> MLVLVAPGQGAQTPGFLTDWLALPGAADRVAAWSDAIGLDLAHFGTKADADEIRDTSVAQPLLVAAGILSAAALGTGFTPGAVAGHSVGEITAAVFAGVLDDTAALSLVRRRGLAMAEAAAVTETGMSALLGGDPEVSVAHLERLGLTPANVNGAGQIVAAGTMEQLAALNEDKPEGVRKVVPLKVAGAFH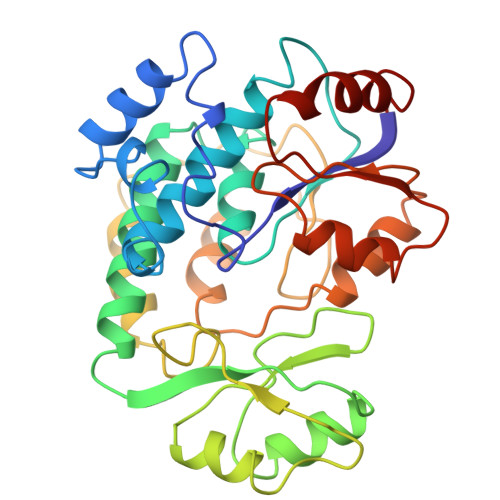TRHMAPAVDKLAEAAKALTPADPKVTYVSNKDGRAVASGTEVLDRLVGQVANPVRWDLCMETFKELGVTAIIEVCPGGTLTGLAKRALPGVKTLALKTPDDLDAARELVAEHT> NLVTPKRELEQGVAFSDLCNFLVTPTVQGWKVYWAGLEFDVNQKGITLLNRLKVNDFAPAWAMTRNLFPHLFKNQQSEVQTPIWALRVILAAGILDQLMDHSLIEPLSGALNLIADWLLTTSTNHFNMRTQRVKDQLSMRMLSLIRSNIINFINKLETLHVVNYKGLLSSVEIGTPSYAIIITRTNMGYLVEVQEPDKSAMDIRHPGPVKFSLLHESTLKPVAT

VP24, one of only eight proteins encoded by ebolaviruses, functions in virus replication and assembly, and is thought to contribute to immune suppression by binding to a certain class of molecules called karyopherins to prevent them from transporting a transcription factor termed STAT1. In addition to its role in interferon antagonism, ebolavirus VP24 has also been proposed to associate with membranes, and is important for assembly and function of the viral ribonucleoprotein complex (RNP), where VP24 binds to the viral nucleoprotein NP. VP24 adopts a compact, single domain, α/β structure of novel fold (DaliLite v.3). The overall shape of VP24 resembles a triangular pyramid of dimensions 73 Å×30 Å×30 Å.

In order to provide 3D templates for understanding VP24 and its many roles in immune evasion, replication and assembly, we crystallized VP24 from Sudan virus (two versions crystallized: SUDV1–233 and SUDV11–233) and Reston virus (one version crystallized: RESTV11–237). We subsequently determined structures of SUDV1–233 and RESTV11–237 by molecular replacement, both at 2.0 Å resolution. Crystal structures presented here include VP24 from an ebolavirus that is pathogenic to humans (Sudan virus; SUDV) and VP24 from an ebolavirus that thus far, appears nonpathogenic to humans (Reston virus; RESTV), although it is lethal to nonhuman primates. The overall folds of SUDV and RESTV VP24 are similar, as expected (r.m.s.d. of 0.81 Å; also see Figure S2b for structural alignment). The entrance to the hydrophobic cavity (11 Å wide) appears to be gated by two residues (Y172 and M71) that point away from each other in RESTV VP24 but toward each other in SUDV VP24, appearing to block the hydrophobic cavity. Crystal packing can sometimes illustrate biologically relevant assemblies, but no tetrameric or other higher oligomeric interactions are observed in crystals of SUDV or RESTV VP24. One pairwise VP24-VP24 interaction is conserved in the crystal packing between the SUDV (P3121) and RESTV VP24 (P1211) structures, although it is currently unclear if it is biologically relevant. This interaction involves α1, β1–3 and the N-terminal region of α8, and buries residue L147 that was previously implicated for virulence, although 142–146 remain solvent exposed. Another crystal lattice interaction observed in both RESTV and SUDV structures involves packing of the hydrophobic N-terminal regions of VP24 into the Face 3 pocket of a neighboring molecule.>GSMSSERVLSYAPAFKSFLDTSFFQELSRLKLDVLKLDSTCQPLTVNLDLHNIPKSADQVPLFLTNRSFEKHNNKRTNEVPLQGSIFNFNVLDEFKNLDKQLFLHQRALECWEDGIKDINKCVSFVIISFADLKKYRFYYWLGVPCFQRPSSTVLHVRPEPSLKGLFSKCQKWFDVNYSKWVCILDADDEIVNYDKCIIRKTKVLAIRDTSTMENVPSALTKNFLSVLQYDVPDLIDFKLLIIRQNEGSFALNATFASI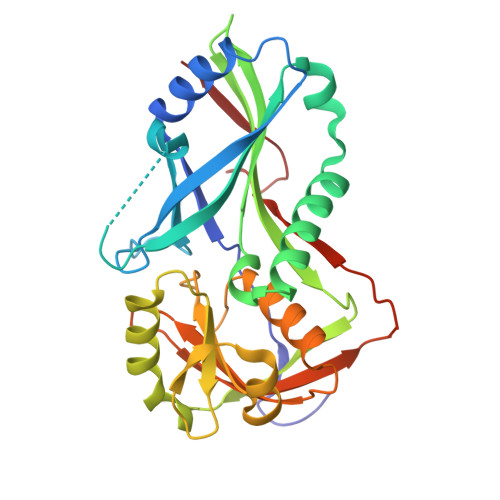DPQSSSSNPDMKVSGWERNVQGKLADRVVDLS[2x]>[2x]MSHPDLNKL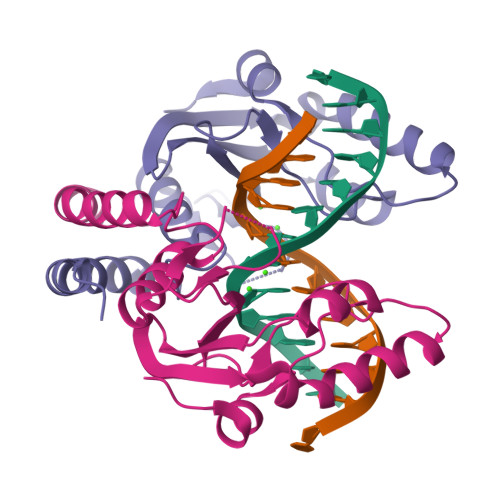LELWPHIQEYQDLALKHGINDIFQDNGGKLLQVLLITGLTVLPGREGNDAVDNAGQEYELKSINIDLTKGFSTHHHMNPVIIAKYRQVPWIFAIYRGIAIEAIYRLEPKDLEFYYDKWERKWYSDGHKDINNPKIPVKYVMEHGTKIY ALLANTOATE ION | C4 H7 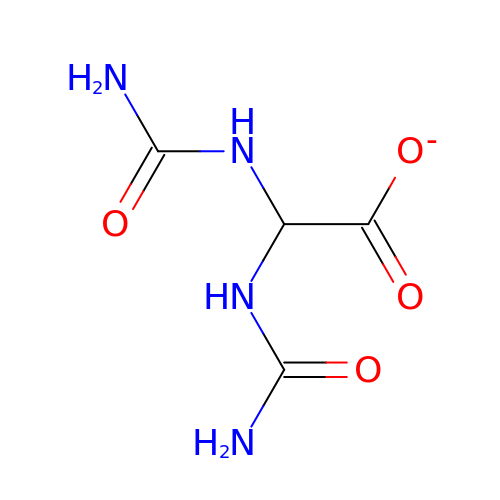N4 O4 | NUCLJNSWZCHRKL-UHFFFAOYSA-M> GSHMTPEAPYASLTEIEHLVQSVCKSYRETCQLRLEDLLRQRSNIFSREEVTGYQRKSMWEMWERCAHHLTEAIQYVVEFAKRLSGFMELCQNDQIVLLKAGAMEVVLVRMCRAYNADNRTVFFEGKYGGMELFRALGCSELISSIFDFSHSLSALHFSEDEIALYTALVLINAHRPGLQEKRKVEQLQYNLELAFHHHLCKTHRQSILAKLPPKGKLRSLCSQHVERMQIFQHLHPIVVQAAFPPLYKELFSTGGSGDHKIIHR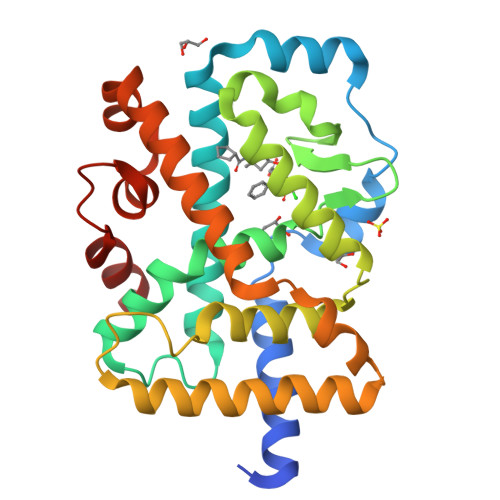LLQEG The HCV NS3/4A protease – a chymotrypsin-like serine protease – is a prime therapeutic target that cleaves four known sites along the virally encoded polyprotein. The NS3/4A protease also hydrolyzes two human proteins, TRIF and MAVS, which are part of the innate immune system, thereby confounding the innate immune response to viral infection. In this study, we report that four chemically representative protease inhibitors – telaprevir, danoprevir, vaniprevir and MK-5172 – exhibit distinct susceptibilities to the protease variants R155K, A156T and D168A. To elucidate the underlying mechanism by which chemically diverse inhibitors bind to the wild-type protease and drug-resistant variants, crystal structures were determined for 16 inhibitor-protease complexes. These complexes include wild-type protease and resistant variants R155K, D168A and A156T each bound to telaprevir, danoprevir, vaniprevir and MK-5172, with resolutions ranging from 1.10–2.50 Å; S139A protease variants were used except for telaprevir, which requires covalent bond formation with the serine 139 for efficient binding.

Relative to the wild type, R155K caused large reductions in potency for danoprevir and vaniprevir, but MK-5172 remained highly active (R155K IC50 = 0.55 nM). Unlike in the danoprevir and vaniprevir complexes with wild type, in the MK-5172-wild-type complex the P2 quinoxaline moiety did not stack on R155 and interacted less with D168 and the electrostatic network involving these residues. Thus, the single-site mutations R155K and D168A only caused very subtle changes in the MK-5172 binding conformations. This subtle effect is reflected in the small loss of potency against the R155K variant; however, MK-5172 exhibited 100-fold lower potency against the D168A variant, likely due to less extensive interactions with D81 and K136 relative to wild-type and R155K. Overall, analysis of the four crystal structures explains MK-5172's significantly retained potency against R155K and D168A as well as its loss of potency against the A156T variant due to the rigidity of the macrocycle. The P2 quinoxaline moiety of MK-5172 stacks against the protease catalytic triad in a novel conformation, explaining its retained potency against R155K and D168A. Unlike other inhibitors, MK5172 does not directly interact with R155 and D168, which mutate to confer multi-drug resistance. This unique binding mode of MK-5172 explains its significantly greater potency against R155K and D168A variants compared to other inhibitors.

>GSHMASMKKKGSVVIVGRINLSGDTAYAQQTRGEEGCQETSQTGRDKNQVEGEVQIVSTATQTFLATSINGVLWTVYHGAGTRTIASPKGPVTQMYTNVDKDLVGWQAPQGSRSLTPCTCGSSDLYLVTRHADVIPVRRRGDSRGSLLSPRPISYLKGSSGGPLLCPAGHAVGIFKAAVSTRGVAKAVDFIPVESLETTMRSP[4x]> MEIDELTALGGLLHDIGKPVQRAGLYSGDHSTQGARFLRDLAENTGRAEYELLSLFSEFHHKGHMKNDELMIRRIKELSPERFGLTMEDVLNALWIVYEADNLASGEREEGQPQASRPLYSVFNPGKAYPWAELDFEKELPVPGDVFSIRSQDYRELVKRLWEELSKAKLRSDRLLPVLEKYLTFVSSVTSEGNIISLYDHMRMTSAIALAMLRAGCTAEDVRSGRCRKEKRFLLIEGDFSGIQDFI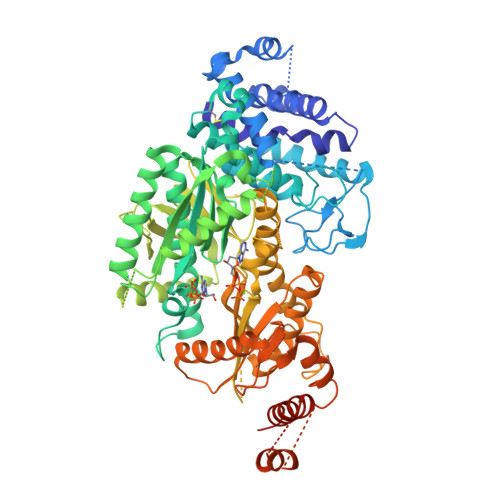YRVSGKGTLKYLRARSAYLELIGWDVVLEILSRLGLTRANVVFNAGGHFMIIAQNTPDAVKELEEIRAKAVEWLYREFESDLYLAIEWEPVSGREFGREGGKNLFAEARKRLKHKLTVRKLKRFGEIKGLFEHGHTERLAECPVCGRELPEGKLEPSASDPETKVCPTCNRLVSLGGNLPKLLGFGRTAKNDAGVLVEGPFSGFVPYLQGGRPVGEQILVKNTLNPGEIPESAQFVPYFVADYFKKDPKGGVAMEFGDYVKRASGIARLGVLRLDVDNLGQAFTHGFMEQGNGKFNTISRTAAFSRMLSLFFRQHINYVLARPKLRPITGDDPARPREATIIYSGGDDVFVVGAWDDVIEFGIELRERFHEFTQGKLTVSAGIGMFPDKYPISVMAREVGDLEDAAKSLPGKNGVALFDREFTFGWDELLSKVIEEKYRHIADYFSGNEERGMAFIYKLLELLAERDDRITKARWVYFLTRMRNPTGDTAPFQQFANRLHQWFQDPTDAKQLKTALHLYIYRTRKEESEHHHHHHHH>[2x]MSYYHHHHHHLESTSLYKAGLTRKFFVGGNWKMNGDYASVDGIVTFLNASADNSSVDVVVAPPAPYLAYAKSKLKAGVLVAAQNCYKVPKGAFTGEISPAMIKDLGLEWVILGHSERRHVFGESDALIAEKTVHALEAGIKVVFCIGEKLEEREAGHTKDVNFR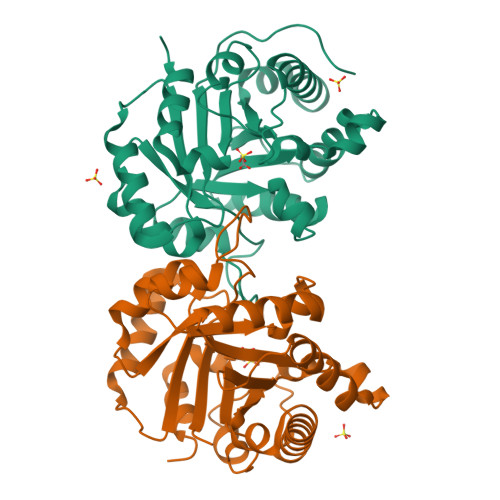QLQAIVDKGVSWENIVIAYEPVWAIGTGKTASGEQAQEVHEWIRAFLKEKVSPAVADATRIIYGGSVTADNAAELGKKPDIDGFLVGGASLKPDFVKIINARSTALSCTCW> GMTLAALCQGVLERLDPRQPGRQLVALSGAPGSGKSTLSNPLAAALSAQGLPAEVVPMDGFHLDNRLLEPRGLLPRKGAPETFDFEGFQRLCHALKHQERVIYPLFDRARDIAIAGAAEVGPECRVAIIEGNYLLFDAPGWRDLTAIWDVSIRLEVPMADLEARL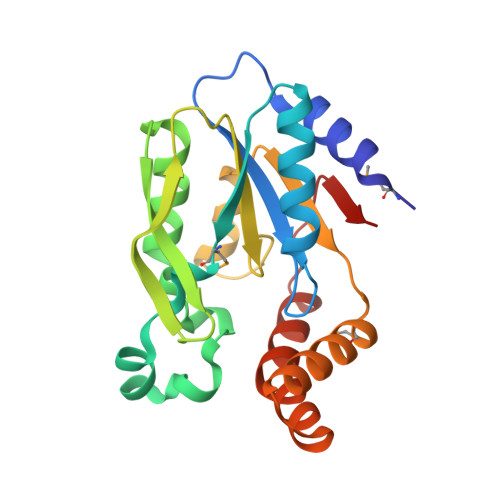VQRWLDHGLNHDAAVARAQGNDLANARAIEAARLPADLTWPQA> AAALSEQLAELEKRSGGRLGVAVLDTATGRRFGYRGDERFPMCSTFKALLAAAVLARVDQGKENLDRRITYGKEDLVDYSPV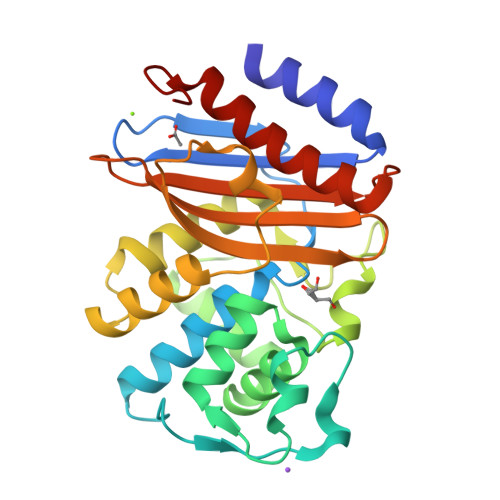TEKHVGDGMTVAELCEAAITYSDNTAANLLLEALGGPAALTAFLRSIGDNVTRLDRWEPELNTAAPGDPRDTTTPAAMAATLRTLLLGDVLSPASRQQLVDWLIANKTGDKRLRAGLPADDRVGDKTGTGEHGTTNDIAVVWPPNHAPIFIAVYLTESQVDADARDAVIAEVARLIVAAWHHHHHH2-ACETYL-THIAMINE DIPHOSPHATE | C14 H21 N4 O8 P2 S | 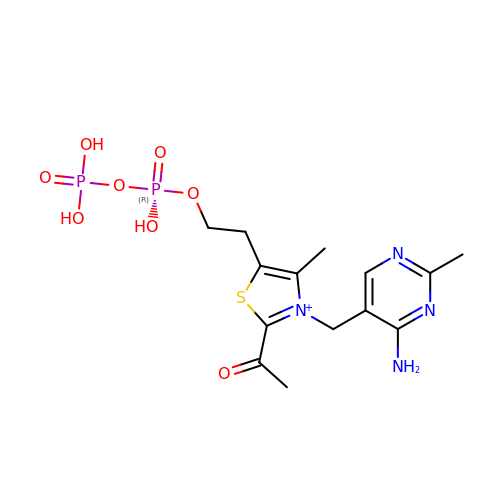GYRGKLZCJRVYRV-UHFFFAOYSA-O>MDTTFGLDLARVETLFKRELRRFDELHPRSAQAYRENRRHWLYGAPLHWMQQWPGNCPLLVKEAQGARVTDIDGQQYVDFALGDSGAMFGHAQPAVADAIARQARRGSTLMLPTEDSLWVGAELARRFGLPYWQVTTSATDANRFVLRLCRMLSGRDKVVVFNCNYHGSVDESQVEFDAAGRMVPRAGVHPNGVRHATTTRLVEFNDLDALEAALAHGDVAAVLTEPFMTNVGMVPPAEGFHAGLRELTRRHDVALIIDETHTISCGPAGYSGAHGLEPDFFVLGACIAGGIPSAVWGCSQAQAERIWAVLPHFRPGQAINHFGFGGTLAGNALQLAAMRATFAEVMTEDAYRHMFQLAAQLEAG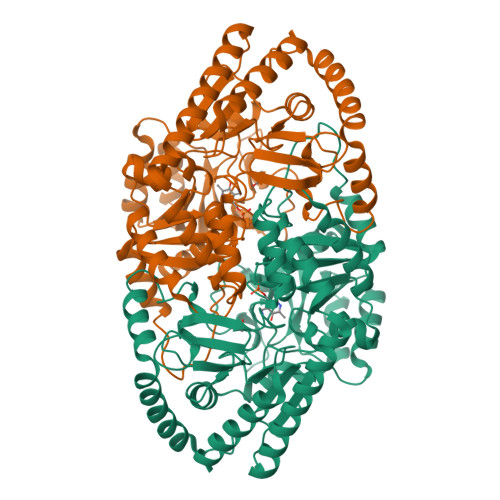VRATLEELRLPWHVTRIGARVEYLFMTHAPRNGGEAHHARNGLIEACLHLYLLNRGVLLTPFHNMALTCPATRAEDVELHDRLLRDCLGELLERPS[2x]>[18x]MTNFLNGVNIGTPGAYAFYQTTQSRPINVEPFRTCYMVGFASNGVNKNVPTRISNLTDFTNVYGTSASTNSVDLFFKNSQGFGNLYFVNVAIPTRYQIVVTAATAGSYSVTVNGVTKAITVVGGATTTTIAADVISAINNDTVLNKEVLATVGGTSSTVVITSKKPTNTTTAAVTGVIFTLTTTTGTSPSVADYVYTINNTFDPALEAGFVIAPEAFSTFTKSDRLSIQVALENLCSAYRYQWAALIDSGAMSEISNTDRAIAEAATYNSVQGHCSYYYPYLINLDDQQVPPSAAVAGMALYRFVIDGFAEPPAGVNFPLKGVKNVAYKVTWEEQNV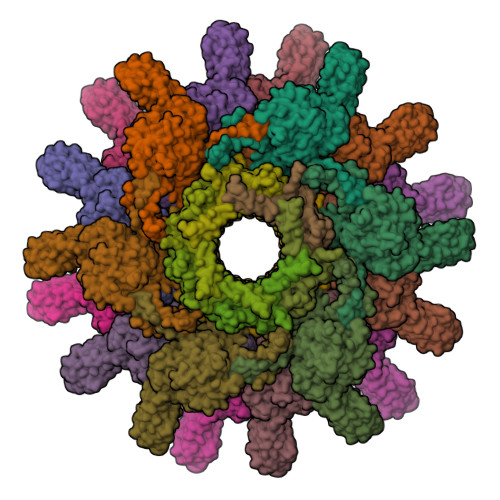ANPEGVNCILNKENYGIVVWGARTLSADPNIVFISTRIILNIVINTLNRGYDFDIFNSVGGTATVLDNIQRKTNTLLTTLYQAGLFYGQTTSEAFSVLGDASVQVPSLLQQGLVNMFIWVVPSTIIERLIINIKQTAIGDLEATVALDTAALQSSVEEGTATEGTAPVV;>MAVSKRPFSINSFAVNLNIGNFVDARYWSKCSKIEKTYNTGEYSDGQSNIIYTLPGAIKYPEVVLSKAFSPGDEELINRLIAVNSDPIAWVTVFIQPMYRDGYYNVPQGGKIILEFCTVARATPINEIDTIGSNAAMFECALNPSRIRSDGGNINWWSEPAAQVAEF[18x]>[2x]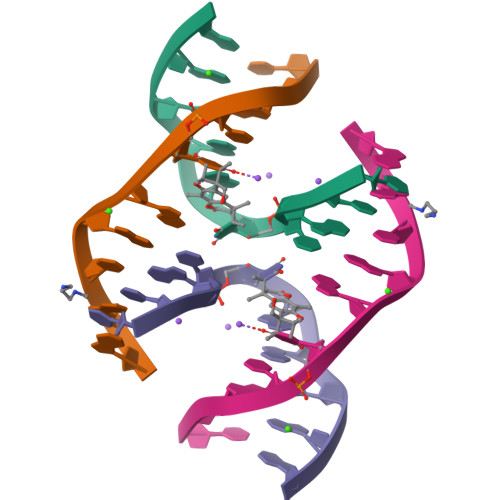CCGCTAGCGG AmyR from E. amylovora is a member of the YbjN family, which have been implicated in regulation of the stress-response in bacteria. Functional studies have previously shown AmyR as an essential regulator of virulence factors in E. amylovora. Importantly, the over-expression of amyR negatively regulates the production of the two E. amylovora exopolysaccharides, amylovoran and levan.

Two different crystal forms developed in the conditions used for crystallisation; rectangular crystals and rhombic plates, with the thicker rectangular crystals regularly producing better diffraction quality crystals. AmyR forms a homodimer in the asymmetric unit with a solvent content of 60.12% (Vm = 3.08 Å3/Da). The protein contains 3 α-helices (residues 10–20; 67–82; 115–138) surrounding a 5 stranded antiparallel β-sheet (residues 34–35; 47–53; 56–64; 88–92; 100–106) with the concave surface facing the solvent and flanked by two protruding loops (residues 27–33; 93–99) to create a channel. Half of the dimer interface is characterized by hydrophobic interactions between the bent α-helix and β-strand of each chain, while the other half of the interaction face forms a hydrophilic pocket containing 18 highly ordered water molecules, and is capped by hydrogen bonding between the two N-terminal tails. The carboxy-terminal 17 amino acids of AmyR form an unstructured chain, accounting for 10% of the protein sequence.

>[2x]GAMGMVSLVVPDLDVLRRWLDQQSITWFECDSCQALHLPHMQNFDGVFDAKIDLMDGVILFSALAEVKPTALIPLAGDLSQINASSLTVKAFLDIQDDNLPKLIVCQSLSAAAGLTYGQFVHFMKESEEQISMIVMEAFANHLLMIAEDEERPPMITSHSLLH>[2x]MAISIKTPEDIEKMRVAGRLAAEVLEMIEPYVKPGVSTGELDRICNDYIVNEQHAVSACLGYHGYPKSVCISINEVVCHGIPDDAKLLKDGDIVNIDVTVIKDGFHGDTSKMFIVGKPTIMGERLCRITQESLYL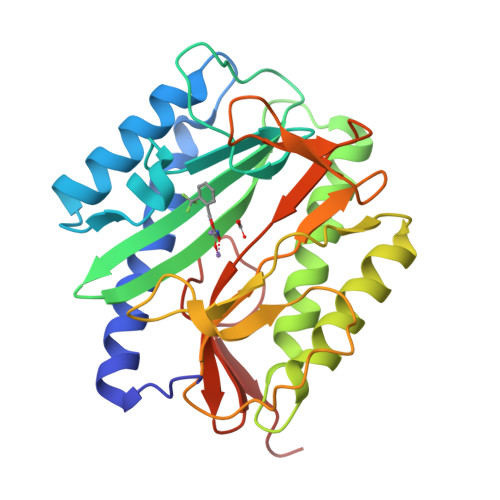ALRMVKPGINLREIGAAIQKFVEAEGFSVVREYCGHGIGRGFHEEPQVLHYDSRETNVVLKPGMTFTIEPMVNAGKKEIRTMKDGWTVKTKDRSLSAQYEHTIVVTDNGCEILTLRKDDTIPAIISHDEA> AVKYYTLEEIQKHNNSKSTWLILHYKVYDLTKFLEEHP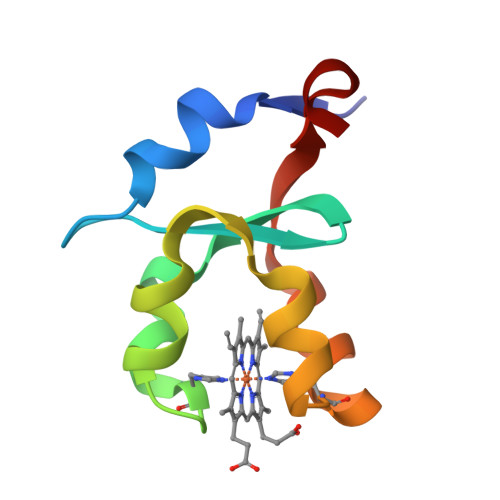GGEEYLREQAGGDATENFEDVGHSTDARELSKTFIIGELHPDDR> 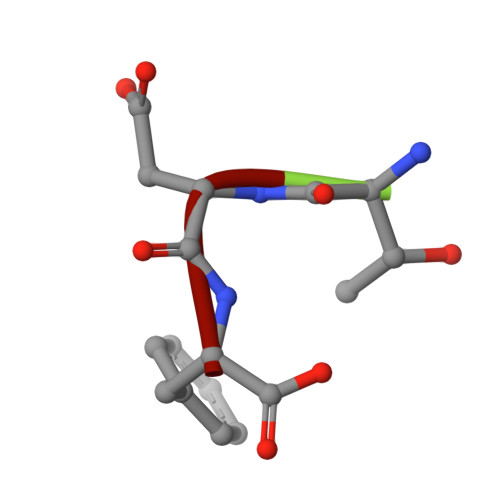TDF>GMTKTAQMIAQQHKDTVAACEAAEAIAIAKDQVWDGEGYTKYTFDDNSVLIQSGTTQYAMDADDADSIKGYAD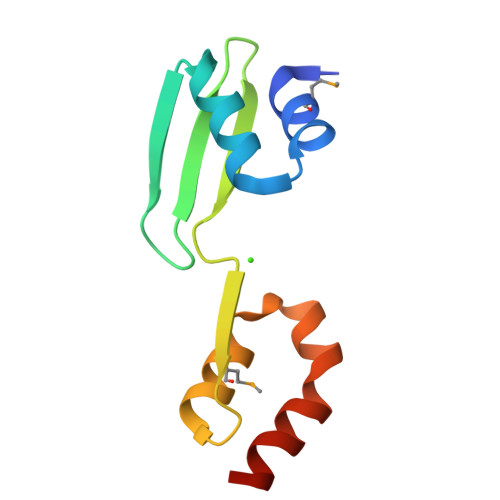WLDDEARSAEASEIERLLESVEEE[2x]>[2x]MELIRF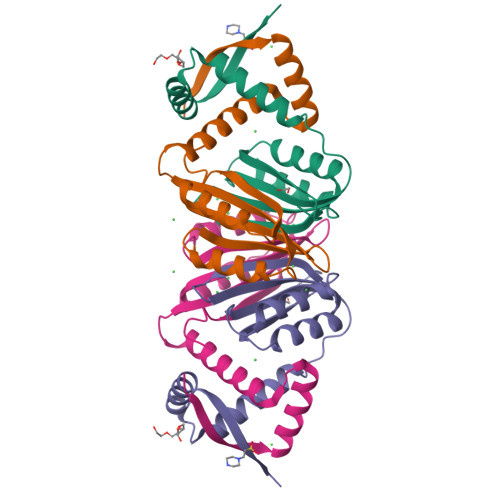SISIPSKLLEKFDQIIEEIGYENRSEAIRDLIRDFIIRHEWEVGNEEVAGTITIVYNHDEGDVVKALLDLQHEYLDEIISSLHVHMDEHNCLEVIVVKGEAKKIKMIADKLLSLKGVKHGKLVMTSTGKELV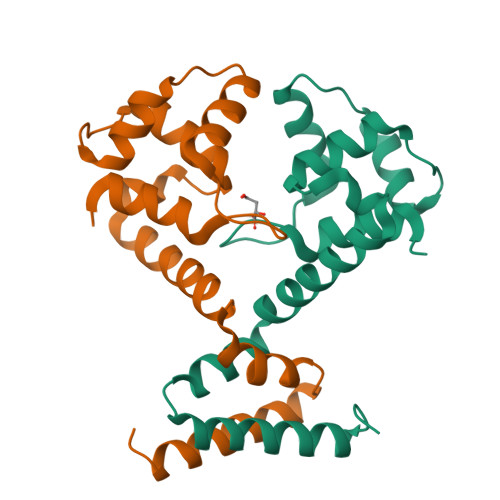>GSSTTFAARLNRLFDTVYPPGRGPHTSAEVIAALKAEGITMSAPYLSQLRSGNRTNPSGATMAALANFFRIKAAYFTDDEYYEKLDKELQWLCTMRDDGVRRIAQRAHGLPSAAQQKVLDRIDELRRAEGIDA[6x]4-(2,3-dihydro-1H-perimidin-2-yl)benzene-1,2-diol | C17 H14 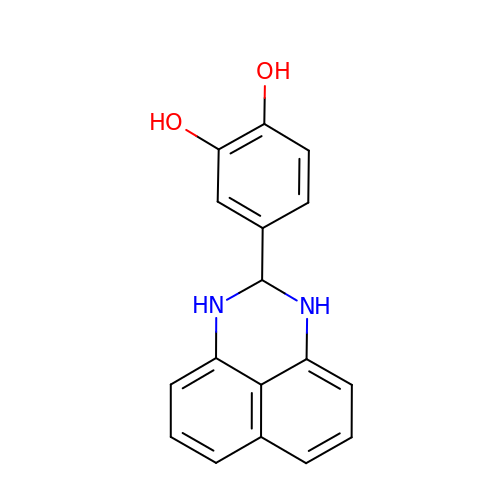N2 O2 | RBGFUFBYYJRGBW-UHFFFAOYSA-N> MNKSQLYPDSPLTDQDFNQLDQTVIEAARRQLVGRRFIELYGPLGRGMQSVFNDIFMESHEAKMDFQGSFDTEVESSRRVNYTIPMLYKDFVLYWRDLEQSKALD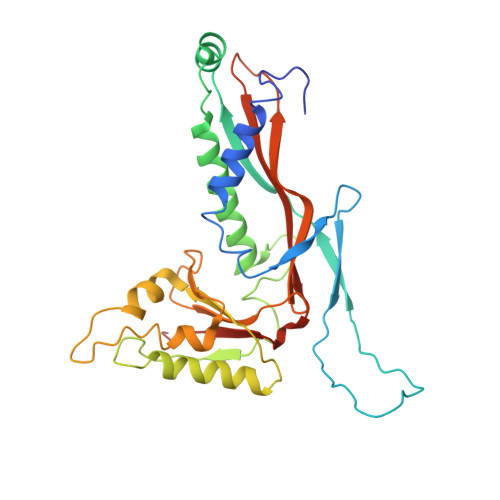IPIDFSVAANAARDVAFLEDQMIFHGSKEFDIPGLMNVKGRLTHLIGNWYESGNAFQDIVEARNKLLEMNHNGPYALVLSPELYSLLHRVHKDTNVLEIEHVRELITAGVFQSPVLKGKSGVIVNTGRNNLDLAISEDFETAYLGEEGMNHPFRVYETVVLRIKRPAAICTLIDPEE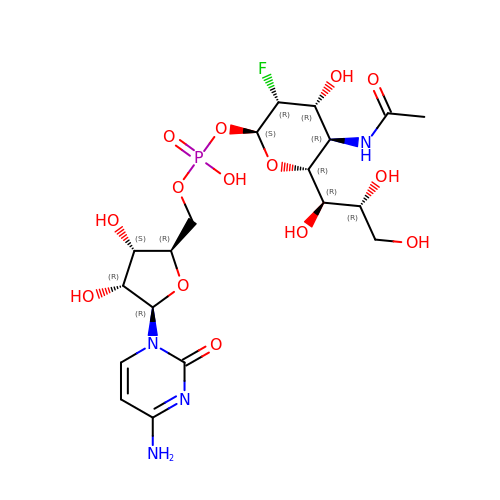CMP-3F(a)-Neu5Ac | C19 H30 F N4 O14 P | DLSXHRIQCIXYOE-DOSPZCANSA-N[CYTIDINE-5'-PHOSPHATE]-BETA-GLUCOSYL-PHOSPHORIC 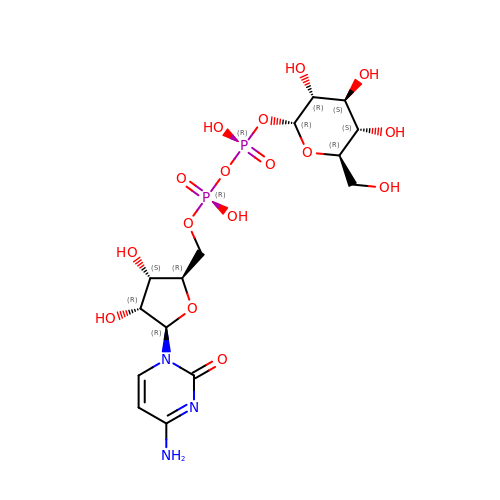ACID ESTER | C15 H25 N3 O16 P2 | CGPHZDRCVSLMCF-JZMIEXBBSA-N The Pfam protein family DUF178 (ID: PF02621) consists of 61 proteins of unknown function, 59 from bacteria and 2 from archaebacteria. Herein, we report the first crystal structures of DUF178 family members, including Q9RXE3 from Deinococcus radiodurans and Q9L0T8 Streptomyces coelicolor and show that they are remarkably similar to Pfam family DUF191. The structure determination of 10093b and 10093f has revealed the unexpected similarity between DUF178 and DUF191 family of proteins suggesting that the information from three-dimensional structures along with the sequence information will predict the family of proteins of similar functions more reliably. We have predicted the protein to be a solute-binding protein based on structure and binding cavity.

The structure of 10093b was determined to 2.5Å resolution using Selenium-SAD. The final refined model of 10093b contains 8 protomers, 18 sulfate ions, and 653 water molecules. Eight monomers A, B, C, D, E, F, G, and H found in the asymmetric unit form four tightly packed dimers (AB, CD, EF, and GH). A dimer interface analysis performed using PDBSUM demonstrated that each pair buries ~3,000Å2 of solvent accessible surface area (12.3% of the total area), a value higher than would be found typically in interacting surfaces for a protein of this size. There are 6 direct hydrogen bonded interactions between the protein atoms across the dimer interface. Such a tight dimer interface suggests that the 10093b dimer is functional, which is supported by the results of analytical gel filtration (data not shown). In the 10093b dimer, Glu172 from the atypical Val166-Ser177 loop makes one of the six hydrogen bonds present in the dimer interface while three other residues in the same loop contribute to van der Waals interactions. We suggest that the atypical loop found in 10093b may help support dimerization. Further analysis of these surface features together with a multiple sequence alignment performed in ClustalW and edited in BioEdit performed for 10093b reveals the presence of most of the conserved residues, including Asn26, Pro47, Ser92, Ser113, Ser116, Ile154, Gly155, and Asp156. The binding pocket of 10093b superposes well with that of nitrate-binding protein. Based on the comparison of structures and binding sites, we predict that this protein could be a solute binding protein, though we cannot at this stage identify the nature of the ion.

>[8x]MSLTNHHPSSTGPQHPYRAGWIHFTNVAPILDSLELPPGVTAITGVPTQMNAALLSGEVDIANVSAVEFIRHADTLAALPDFSVAVLGPVYSVNLFHTCPLPELRRVALTSQSAMSVALLEVLLRQKGLSPVLERAEGTAESLLAAGYDGVLRIGDDALREWYGVVGPLTPERTMTSLPHTGRGITVTDLAQEWFDLTGHPFTFAVWAYRKDNPPPAALLQAMREARRRGIGHLAEVSQRHAEKLGLPERVVQHYLWNFRYHLEAPDRLGLREFADLAVPGHAELTFGAREEAEGHHHHHH> SMKGSGQIQLWQFLLELLADRANAGCIAWEGGHGEFKLTDPDEVARRWGERKSKPNMNYDKLSRALRYYYDKNIMSKVHG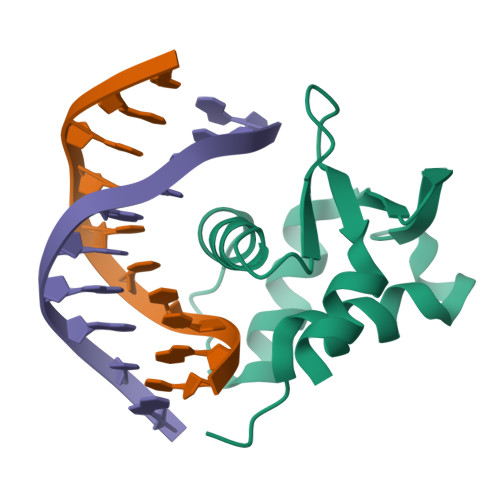KRYAYRFDFQGLAQACQPPPAH>MANYFNTLNLRQQLAQLGKCRFMGRDEFADGASYLQGKKVVIVGCGAQGLNQGLNMRDSGLDISYALRKEAIAEKRASWRKATENGFKVGTYEELIPQADLVINLTPDKQHSDVVRTVQPLMKDGAALGYSHGFNIVEVGEQIRKDITVVMVAPKCPGTEVREEYKRGFGVPTLIAVHPENDPKGEGMAIAKAWAAATGGHRAGVLESSFVAEVKSDLMGEQTILCGMLQAGSLLCFDKLVEEGTDPAYAEKLIQFGWETITEALKQGGITLMMDRLSNPAKLRAYALSEQLKEIMAPLFQKHMDDIISGEFSSGMMADWANDDKKLLTWREETGKTAFETAPQYEGKIGEQEYFDKGVLMIAMVKAGVELAFETMVDS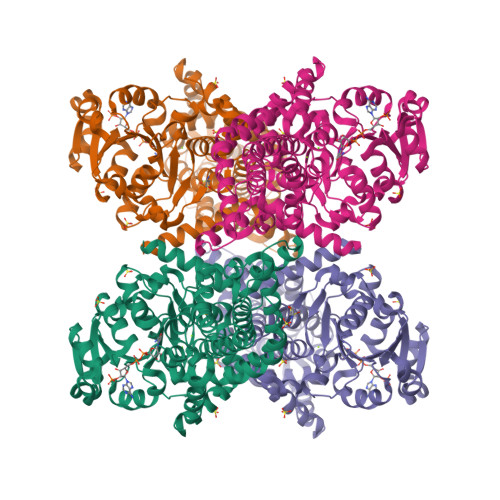GIIEESAYYESLHELPLIANTIARKRLYEMNVVISDTAEYGNYLFSYACVPLLKPFMAELQPGDLGKAIPEGAVDNGQLRDVNEAIRSHAIEQVGKKLRGYMTDMKRIAVAG[2x]> TQEIYPIKEANGRTRKALIICNTEFKHLSLRYGANFDIIGMKGLLEDLGYDVVVKEELTAEGMESEMKDFAALSEHQTSDSTFLVLMSHGT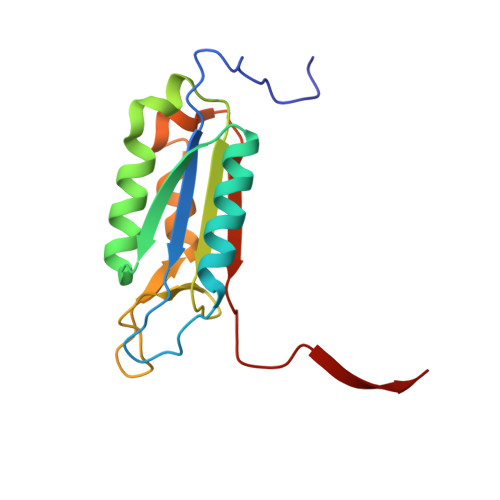LHGICGTMHSEKTPDVLQYDTIYQIFNNCHCPGLRDKPKVIIVQAARGGNSGEMWIRE>MRGSHHHHHHGLVPRGSMIRTMLQGKLHRVKVTHADLHYEGTCAIDQDFLDAAGILE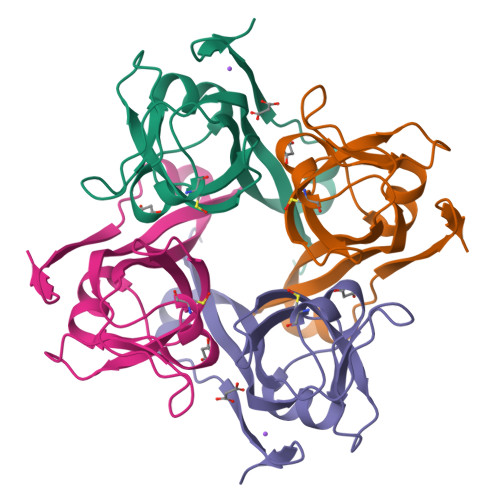NEAIDIWNVTNGKRFSTYAIAAERGSRIISVNGAAAHCASVGDIVIIASFVTMPDEEARTWRPNVAYFEGDNEMKRTAKAIPVQVA[2x]>KLPYKVADIGLAAWGRKALDIAENEMPGLMRMRERYSASKPLKGARIAGCLHMTVETAVLIETLVTLGAEVQWSSCNIFSTQDHAAAAIAKAGIPVYAWKGETDEEYLWCIEQTLYFKDGPLNMILDDGGDLTNLIHTKYPQLLPGIRGISEETTTGVHNLYKMMANGILKVPAINVNDSVTKSKFDNLYGCRESLIDGIKRATDVMIAGKVAVVAGYGDVGKGCAQALRGFGARVIITEIDPINALQAAMEGYEVTTMDEACQEGNIFVTTTGCIDIILGRHF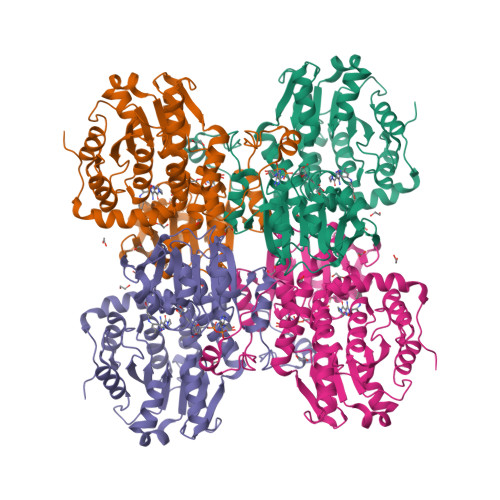EQMKDDAIVCNIGHFDVEIDVKWLNENAVEKVNIKPQVDRYRLKNGRRIILLAEGRLVNLGCAMGHPSFVMSNSFTNQVMAQIELWTHPDKYPVGVHFLPKKLDEAVAEAHLGKLNVKLTKLTEKQAQYLGMSCDGPFKPDHYRY[2x]>MGHHHHHHFNEVHSSHGHTLLLITKPSLQATALLQHLKQSLAITGKLHNIQRSLEDISAGCIVLMDMME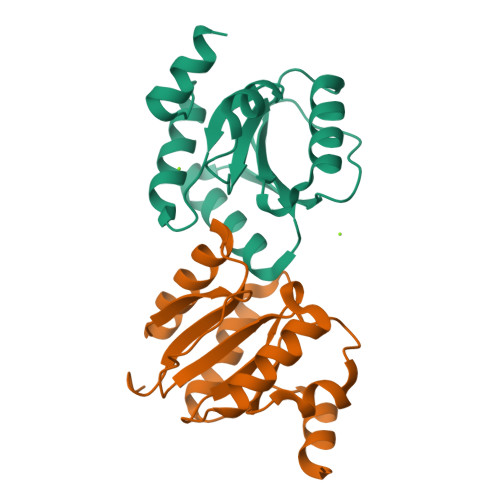ADKKLIHYWQDNLSRKNNNIKTLLLNTPDDYPYREIENWPHINGVFYATEDQEHVVSGLQGILRGECYFSQKLASYLITHSGNYRY[2x]>MKVLVINAGSSSLKYQLIDMTNESALAVGLCERIGIDNSIITQKKFDGKKLEKLTDLPTHKDALEEVVKALTDDEFGVIKDMGEINAVGHRVVHGGEKFTTSALYDEGVEKAIKDCFELAPLHNPPNMMGISACAEIMPGTPMVIVFDTAFHQTMPPYAYMYALPYDLYEKHGVRKYGFHGTSHKYVAERAALMLGKPAEETKIITCHLGNGSSITAVEGGKSVETSMGFTPLEGLAMGTRCGSID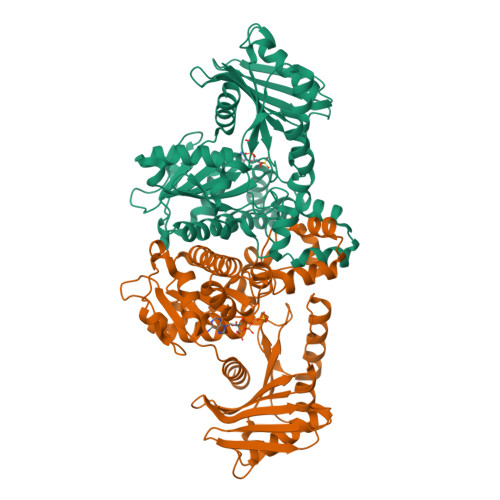PAIVPFLMEKEGLTTREIDTLMNKKSGVLGVSGLSNDFRDLDEAASKGNRKAELALEIFAYKVKKFIGEYSAVLNGADAVVFTAGIGENSASIRKRILTGLDGIGIKIDDEKNKIRGQEIDISTPDAKVRVFVIPTNEELAIARETKEIVETEVKLRSSIPV[2x]> STIPSEIINWTILNEIISMDDDDSDFSKGLIIQFIDQAQTTFAQMQRQLDGEKNLTEL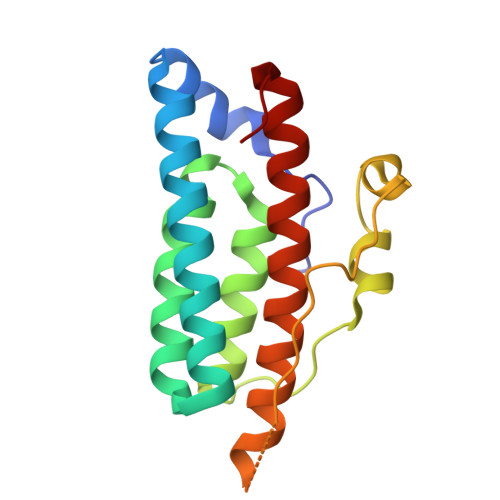DNLGHFLKGSSAALGLQRIAWVCERIQNLGRKMEHFFPNKTELVNTLSDKSIINGINIDEDDEEIKIQVDDKDENSIYLILIAKALNQSRLEFKLARIELSKYYNTNL>[2x]ETGELKIECPHTIGLGQGLVIGSVELPPVPL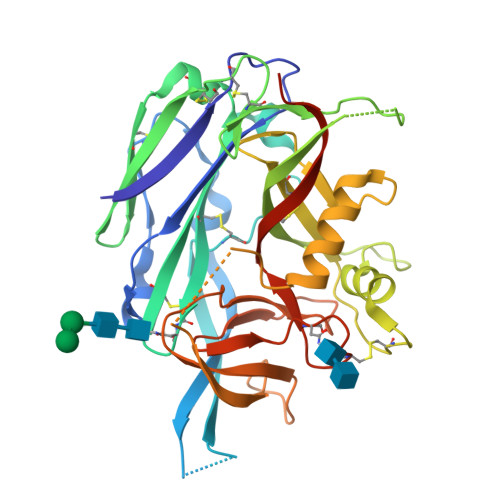TQVESLKLESSCNFDLHTSTSSQQPFTKWTWEMKSDLAENTQASSTSFQTKSSEINLRGLCLVPPLVIETAARTRKTIACFDLSCNQTACQPTVFLIGPIQTCITTKSCLLGLGDQRIQVNYEKTYCVSGQLVEGVCFNPVHTMALSQPSHTYDIVTVMVRCFLIAKKVSTGDSMKLEKSFETLVQKTSCTGNGFQGYYICLVGSSSEPLYIPTLDDYRSAEVLSRMAFAPHGEDHDVEKNAISAMRIIGKVTGKAPSTESSDTIQGVAFSGNPLYTSTGVLTAKDDPVYIWAPGIIMEGNHSVCDKKTLPLTWTGFIPLPGEIEKTGTKHHHHHH> MAHHHHHHSSGLEVLFQGPSGIVPQLQNIVSTVNLGCKLDLKTIALRARNAEYNPKRFAAVIMRIREPRTTALIFSSGKMVCTGAKSEEQSRLAARKYARVVQKLGFPAKFLDFKIQNMVGSCDVKFPIRLEGLVLTHQQFSS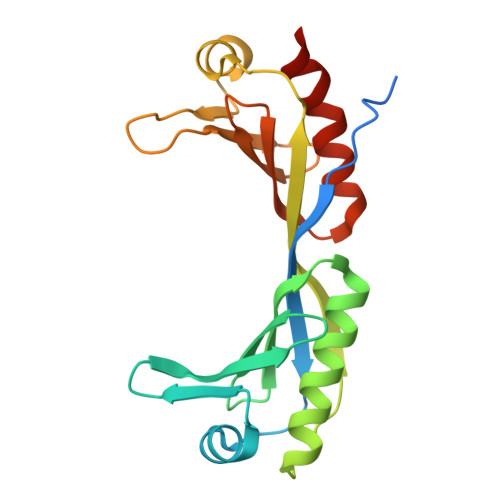YEPELFPGLIYRMIKPRIVLLIFVSGKVVLTGAKVRAEIYEAFENIYPILKGFRKTT>AMLPHGLIVSCQALPDEPLHSSFIMSKMALAAYEGGAVGIRANTKEDILAIKETVDLPVIGIVKRDYDHSDVFITATSKEVDELIESQCEVIALDATLQQRPKETLDELVSYIRTHAPNVEIMADIATVEEAKNAARLGFDYIGTTLHGYTSYTQGQLLYQNDFQFLKDVLQSVDAKVIAEGNVITPDM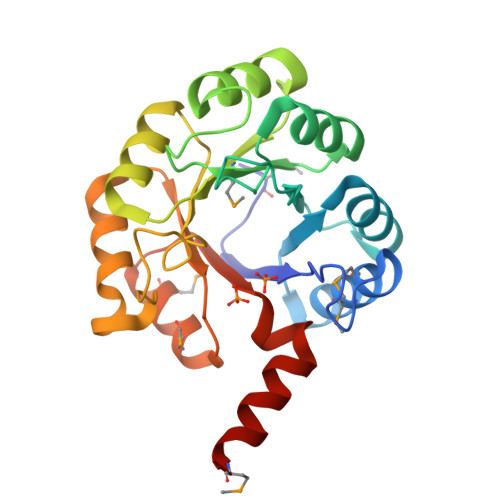YKRVMDLGVHCSVVGGAITRPKEITKRFVQVMED[2x]>[2x]GPGSMVSLEGKVALITGAGSGFGEGMAKRFAKGGAKVVIVDRDKAGAERVAGEIGDAALAVAADISKEADVDAAVEAALSKFGKVDILVNNAGIGHKPQNAELVEPE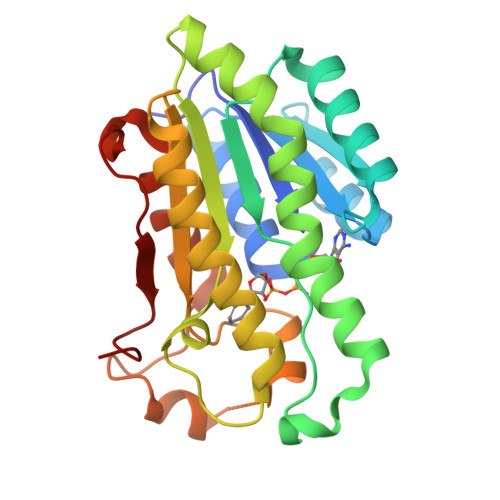EFDRIVGVNVRGVYLMTRKLIPHFKENGAKGQECVILNVASTGAGRPRPNLAWYNATKGWVVSVTKALAIELAPAKIRVVALNPVAGETPLLTTFMGEDSEEIRKKFRDSIPMGRLLKPDDLAEAAAFLCSPQASMITGVALDVDGGRSI>[2x]MTPIE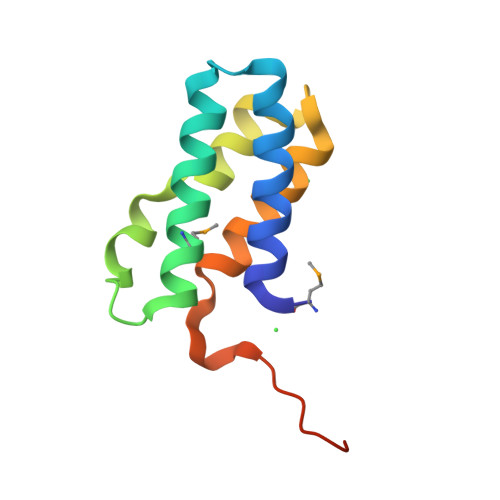YIDRALALVVDRLARYPGYEVLLSAEKQLQYMRSVLLDRSLDRSALHRLTLGSIAVKEFDETDPELSRALKDAYYVGIRTGRGLKVDLPLEHHHHHH> MAAVAAVAARRRRSWASLVLAFLGVCLGITLAVDRSNFKTCEESSFCKRQRSIRPGLSPYRALLDSLQLGPDSLTVHLIHEVTKVLLVLELQGLQKNMTRFRIDELEPRRPRYRVPDVLVADPPIARLSVSGRDENSVELTMAEGPYKIILTARPFRLDLLEDRSLLLSVNARGLLEFEHQRAPRVSQGSKDPAEGDGAQPEETPRDGDKPEETQGKAEKDEPGAWEETFKTHSDSKPYGPMSVGLDFSLPGMEHVYGIPEHADNLRLKVTEGGEPYRLYNLDVFQYELYNPMALYGSVPVLLAHNPHRDLGIFWLNAAETWVDISSNTAGKTLFGKMMDYLQGSGETPQTDVRWMSETGIIDVFLLLGPSISDVFRQYASLTGTQALPPLFSLGYHQSRWNYRDEADVLEVDQGFDDHNLPCDVIWLDIEHADGKRYFTWDPSRFPQPRTMLERLASKRRKLVAIVDPHIKVDSGYRVHEELRNLGLYVKTRDGSDYEGWCWPGSAGYPDFTNPTMRAWWANMFSYDNYEGSAPNLFVWNDMNEPSVFNGPEVTMLKDAQHYGGWEHRDVHNIYGLYVHMATADGLRQRSGGMERPFVLARAFFAGSQRFGAVWTGDNTAEWDHLKISIPMCLSLGLVGLSFCGADVGGFFKNPEPELLVRWYQMGAYQPFFRAHAHLDTGRREPWLLPSQHNDIIRDALGQRYSLLPFWYTLLYQAHREGIPVMRPLWVQYPQDVTTFNIDDQYLLGDALLVHPVSDSGAHGVQVYLPGQGEVWYDIQSYQKHHGPQTLYLPVTLSSIPVFQRGGTIVPRWMRVRRSSECMKDDPITLFVALSPQGTAQGELFLDDGHTFNYQTRQEFLLRRFSFSGNTLVSSSADPEGHFETPIWIERVVIIGAGKPAAVVLQTKGSPESRLSFQHDPETSVLVLRKPGINVASDWSIHLR;> MLLPLLLLLPMCWAVEVKRPRGVSLTNHHFYDESKPFTCLDGSATIPFDQVNDDYCDCKDGSDEPGTAACPNGSFHCTNTGYKPLYIPSNRVNDGVCDCCDGTDEYNSGVICENTCKEKGRKERESLQQMAEVTREGFRLKKILIEDWKKAREEKQKKLIELQAGKKSLEDQVEMLRTVKEEAEKPEREAKEQHQKLWEEQLAAAKAQQEQELAADAFKELDDDMDGTVSVTELQTHPELDTDGDGALSEAEAQALLSGDTQTDATSFYDRV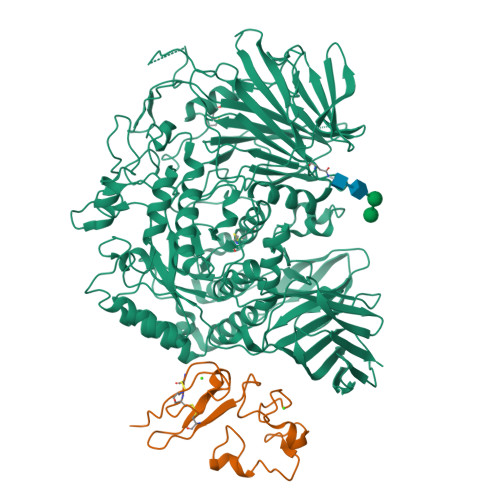WAAIRDKYRSEALPTDLPAPSAPDLTEPKEEQPPVPSSPTEEEEEEEEEEEEEAEEEEEEEDSEEAPPPLSPPQPASPAEEDKMPPYDEQTQAFIDAAQEARNKFEEAERSLKDMEESIRNLEQEISFDFGPNGEFAYLYSQCYELTTNEYVYRLCPFKLVSQKPKLGGSPTSLGTWGSWIGPDHDKFSAMKYEQGTGCWQGPNRSTTVRLLCGKETMVTSTTEPSRCEYLMELMTPAACPEPPPEAPTEDDHDEL5-[(4-{trans-4-hydroxy-4-[3-(trifluoromethyl)phenyl]cyclohexyl}piperazin-1-yl)methyl]pyridin-2(1H)-one | C23 H28 F3 N3 O2 | 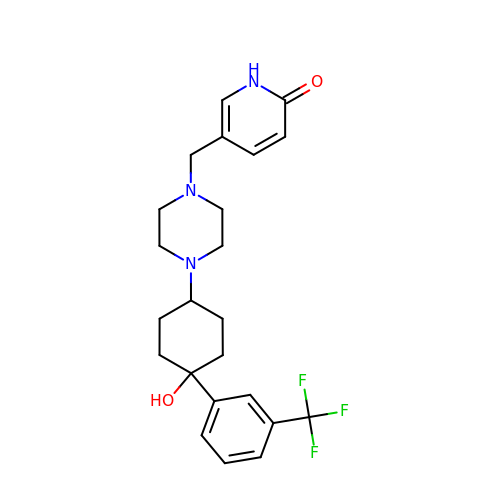HGNRFWCPFKHVCH-AQYVVDRMSA-N We report that T. vaginalis has acquired, by lateral gene transfer from bacteria, genes encoding peptidoglycan hydrolases of the NlpC/P60 family. NlpC_A1 and NlpC_A2 consist of the C-terminal NlpC/P60 domain preceded by two bacterial SH3 domains. The NlpC/P60 domain adopts the classical papain-like fold, with a central β-sheet of 5 strands displaying an antiparallel arrangement. Hence, we concluded that NlpC_A1 and NlpC_A2 are dl-endopeptidases with specificity for the tetrapeptides in peptidoglycan and with greater activity toward monomeric muropeptides.

The structures of NlpC_A1 T. vaginalis AG_119910 (TVAG_119910) and NlpC_A2 (TVAG_457240) were determined by X-ray crystallography. The similarity to other NlpC proteins allows us to assign the active-site residues of Cys179-His234-His246, present in all TvNlpC/P60 sequences. The active-site cysteine is located at the N terminus of helix α3, while the two histidines are in strands β15 and β16. The active-site residues sit in a “T”-shaped groove that is bounded by strands β14 and β15 in the NlpC domain, with the cross of the T formed by the β3 strand in the first SH3b domain. A surface electrostatic calculation demonstrated that the slightly positively charged active-site groove carries two pronounced areas of strong positive charge. The first of the two areas is adjacent to the catalytic cysteine, and the second is at the base of a small pocket at the interface between the NlpC domain and the first SH3b domain bounded by the residues His195, Tyr43, Trp44, Tyr46, Phe193, and Gln184. As expected, mutation of the catalytic Cys179 to either Ser or Ala in NlpC_A1 and NlpC_A2 completely abolished their activity toward PG.

> GPGMLSILLSASSSYQTQTIGRLTTPGTNLVKAYKSSNPDLARNCYWLYFDYYVHILGYENGFAHVRIGTEDCWISKDSLEEITIPTQSVTEANIYSEPSRTGTIVRYVPANSQVTILDFNCDGFYRINYRGYIGYILEDALQYKWKQIDGANDGERAANLVKTKLGCKYILGMSGPDTYDCSGLMQWAYNRLDIFMHRTADVQDLHGQLIEDAQDILPGDIITFRTDSDNPMLVTHVGMYVGNGQFIHASTNGYVVKYQDFYKYPYPVSTIRRYWTK Ribonuclease E (RNase E) is a metal-dependent hydrolytic enzyme that cleaves polymeric ribonucleic acid internally and serves as a central element in RNA metabolism of diverse bacteria. The NTD of RNase E (1–529) is highly conserved and harbors the catalytic activity of the enzyme. RNase E forms a tetramer in which the protomers are arranged as a dimer of dimers and accommodate an RNA substrate at the active site formed by the interface of two subunits of the principal dimer unit. The catalytic site is located in a DNase I-like domain, where conserved acidic groups D303 and D346 coordinate the magnesium ions that assist in the hydrolytic attack of single-stranded RNA.

To identify additional RNA-enzyme interaction sites within the NTD of RNase E, co-crystallizations were undertaken of the complex of full-length sRNA RprA with the catalytically inactive RNase E (1–510) D303R, D346R. Diffraction data were collected from tens of specimens prepared under different buffer conditions, and the highest resolution obtained was 3.95 Å. Crystals of the complex were dissolved and analyzed on a denaturing RNA gel, revealing the full-length RNA present (data not shown). It is likely that only small portions of the RNA could be modeled into the map due to a combination of low resolution and structural disorder. The duplex binding region is formed by a surface presented by the RNase H domain of one protomer and the small domain of the partner protomer that forms the principal dimer (i.e., the dimer unit of the dimer of dimers within the tetramer). At the limited resolution of the crystal structure, it is not possible to confidently identify amino acid interactions with the duplex. Thus, the complex of the RNA duplex with RNase E identified in the crystal structures with RprA and SdsR sRNAs revealed a surface of 8 amino acids of RNase E that could potentially interact with the RNA, namely R3, Q22, H268, Y269, Q270 (from the RNase H domain), K433, R488, and R490 (from the small domain). The RprA used in the crystallization had a 5′ monophosphate, which is required for its efficient processing by RNase E (data not shown), and is probably engaging in the 5′ binding pocket of the enzyme where it provides allosteric activation. The identified duplex binding surface comprises a relatively large area, with binding defined between the protein and RNA backbone rather than particular bases. Such a mechanism ensures lack of sequence specificity, but structure specificity: upon stable binding of the stem, if any single-stranded regions are present in the RNA, these can be aligned in the active site.

>[4x]MKRMLINATQQEELRVALVDGQRLYDLDIESPGHEQKKANIYKGKITRIEPSLEAAFVDYGAERHGFLPLKEIAREYFPANYSAHGRPNIKDVLREGQEVIVQIDKEERGNKGAALTTFISLAGSYLVLMPNNPRAGGISRRIEGDDRTELKEALASLELPEGMGLIVRTAGVGKSAEALQWDLSFRLKHWEAIKKAAESRPAPFLIHQESNVIVRAFRDYLRQDIGEILIDNPKVLELARQHIAALGRPDFSSKIKLYTGEIPLFSHYQIESQIESAFQREVRLPSGGSIVIDSTEALTAIRINSARATRGGDIEETAFNTNLEAADEIARQLRLRDLGGLIVIRFIDMTPVRHQRAVENRLREAVRQDRARIQISHISRFGLLEMSRQRLSPSLGESSHHVCPRCSGTGTVRDNESLSLSILRLIEEEALKENTQEVHAIVPVPIASYLLNEKRSAVNAIETRQDGVRCVIVPNDQMETPHYHVLRVRKGEETPTLSYMLPKLHEEAM(3R,4S,5R)-5-{[(1R)-1-CARBOXY-2-FLUORO-1-(PHOSPHONOOXY)ETHYL]OXY}-4-HYDROXY-3-(PHOSPHONOOXY)CYCLOHEX-1-ENE-1-CARBOXYLIC 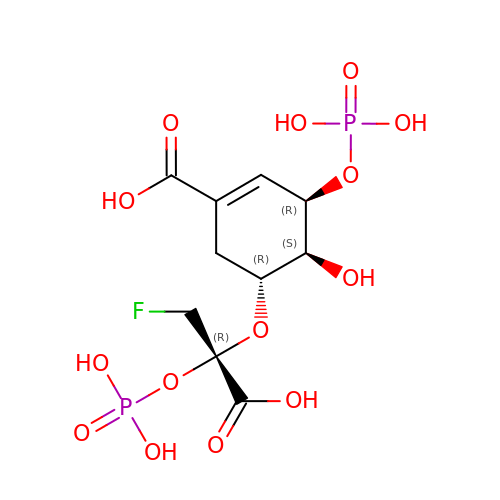ACID | C10 H15 F O14 P2 | HTMVUWTXBMZROV-JQCUSGDOSA-N4-{[(1R,2S)-2-fluoro-2-methylcyclopentyl]amino}pyrrolo[1,2-b]pyridazine-3-carboxamide 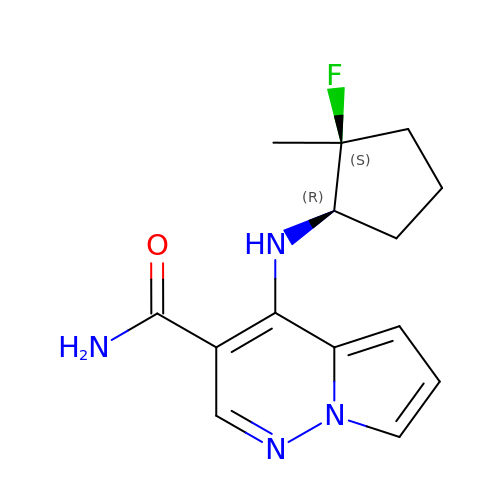| C14 H17 F N4 O | UPBRYBJZTWHUQK-RISCZKNCSA-N> MSSWDRFDTPWDSIIDESTWEHYTFKYDASFEAFSSMEVDEDLTITVSVLFASTSDNTVTVGQVLGLTMDNRAGSYFGAGSSWTSEA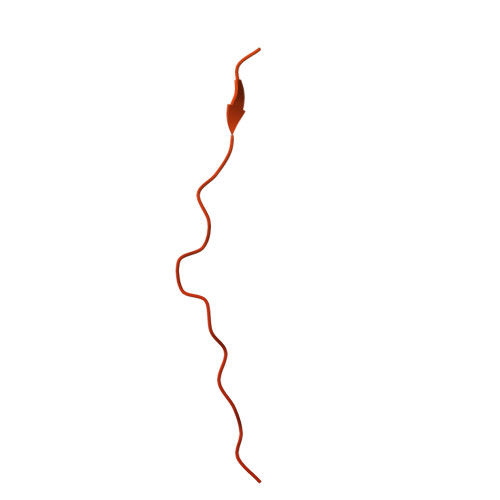AVNNEAGSGFQSSHALQLSYSVEDGVISSFGSEAFCSFYNTVSFESSSDVQAAVNSLYNLDVLFSSGSGDSEQHYVVFGETASFESLAEHETSSQYITHVECMFNSVVEFEVKTYDWGRPVKPVGSDWSTDTPVVGVWVNEIYNGNKDWGES>[2x]MGNGQGRDWKMAIKRC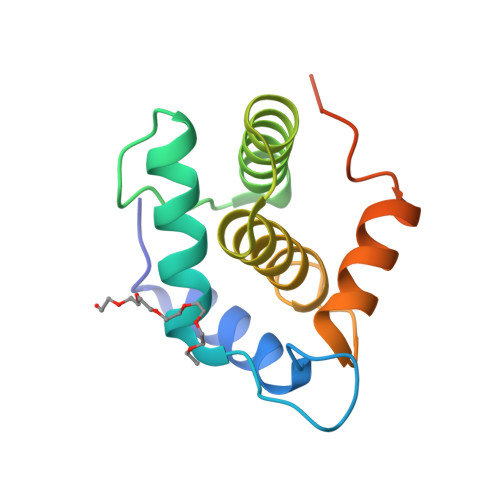SNVAVGVGGKSKKFGEGNFRWAIRMANVSTGREPGDIPETLDQLRLVICDLQERREKFGSSKEIDMAIVTLKVFAVAGLLNMTVSTAAAAENMYSQMGLDTRPSLVPRGSLEHHHHHH> MFENITTAPADPILGLADLLRADERPGKIDLGMGVYNDETGKTPVLTSVKKAEQYLLENETTKNYLGIDGIPEFGRCTQELLFGKGSALINDKRARTAQTPGGTGALRVAADFLAKNTSVKRVWVSNPGWPTHKSVFNSAGLEVREYAYYDAENHTLDFDALINSLNEAQAGDVVLFHGCCHNPTGIDPTLEQWQTLAQLSVEKGWLPLFDFAYQGFARGLEEDAEGLRAFAAMHKELIVASSYSKNFGLYNERVGACTLVAADSETVDRAFSQMKAAIRVNYSSPPAHGASVVATILSNDALRAIWEQELTDMRQRIQRMRQLFVNTLQEKGANRDFSFTIKQNGMFFFGGLTKEQVLRLREEFGVYAVASGRLNVAGMTPDNLAPLC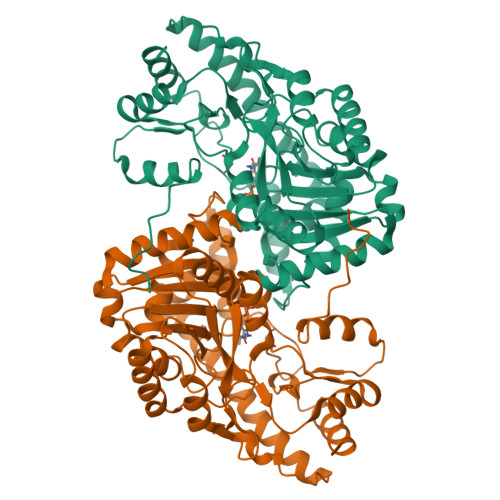EAIVAVL N-HYDROXY-L-ARGININAMIDE | C6 H15 N5 O2 | 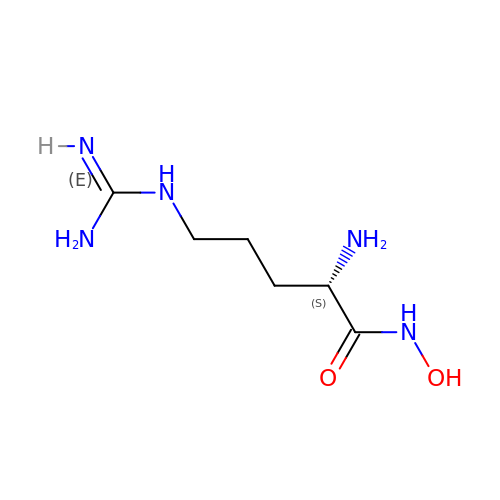IXHTVNGQTIZAFS-BYPYZUCNSA-N>[14x]XGE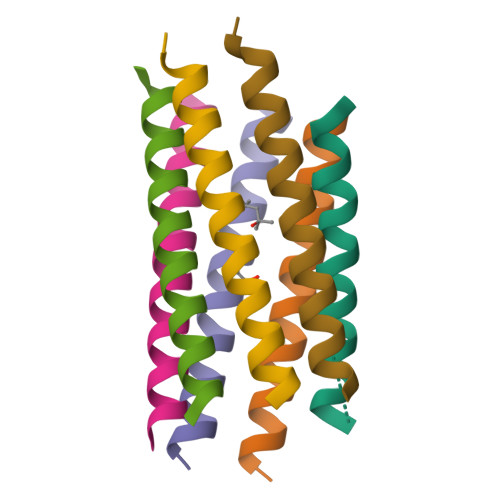LAQSIKELAKSIKEEAWSIKELAQSIKGX>GAMAPPTLPPYFMKGSIIQLANGELKKVEDLKTEDFIQSAEISNDLKIDSSTVERIEDSHSPGVAV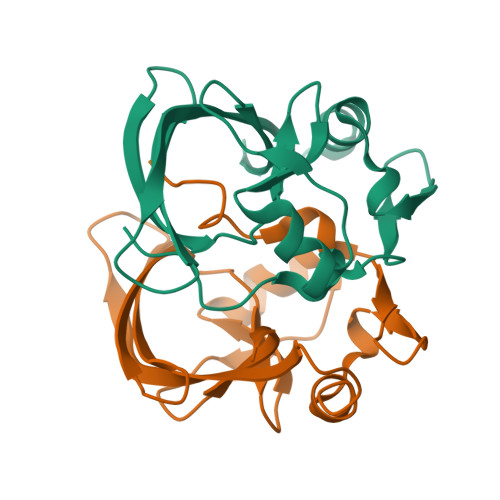IQFAVGEHRAQVSVEVLVEYPFFVFGQGWSSCCPERTSQLFDLPCSKLSVGDVCISLTLK[4x]> MDYKDDDDKLAAANSSIDLISTSLYKKAGLTMVTGGGAAPPGTVTEPLPSVIVLSAGRKMAAAAAAASGPGCSSAAGAGAAGVSEWLVLRDGCMHCDADGLHSLSYHPALNAILAVTSRGTIKVIDGTSGATLQASALSAKPGGQVKCQYISAVDKVIFVDDYAVGCRKDLNGILLLDTALQTPVSKQDDVVQLELPVTEAQQLLSACLEKVDISSTEGYDLFITQLKDGLKNTSHETAANHKVAKWATVTFHLPHHVLKSIASAIVNELKKINQNVAALPVASSVMDRLSYLLPSARPELGVGPGRSVDRSLMYSEANRRETFTSWPHVGYRWAQPDPMAQAGFYHQPASSGDDRAMCFTCSVCLVCWEPTDEPWSEHERHSPNCPFVKGEHTQNVPLSVTLATSPAQFPCTDGTDRISCFGSGSCPHFLAAATKRGKICIWDVSKLMKVHLKFEINAYDPAIVQQLILSGDPSSGVDSRRPTLAWLEDSSSCSDIPKLEGDSDDLLEDSDSEEHSRSDSVTGHTSQKEAMEVSLDITALSILQQPEKLQWEIVANVLEDTVKDLEELGANPCLTNSKSEKTKEKHQEQHNIPFPCLLAGGLLTYKSPATSPISSNSHRSLDGLSRTQGESISEQGSTDNESCTNSELNSPLVRRTLPVLLLYSIKESDEKAGKIFSQMNNIMSKSLHDDGFTVPQIIEMELDSQEQLLLQDPPVTYIQQFADAAANLTSPDSEKWNSVFPKPGTLVQCLRLPKFAEEENLCIDSITPCADGIHLLVGLRTCPVESLSAINQVEALNNLNKLNSALCNRRKGELESNLAVVNGANISVIQHESPADVQTPLIIQPEQRNVSGGYLVLYKMNYATRIVTLEEEPIKIQHIKDPQDTITSLILLPPDILDNREDDCEEPIEDMQLTSKNGFEREKTSDISTLGHLVITTQGGYVKILDLSNFEILAKVEPPKKEGTEEQDTFVSVIYCSGTDRLCACTKGGELHFLQIGGTCDDIDEADILVDGSLSKGIEPSSEGSKPLSNPSSPGISGVDLLVDQPFTLEILTSLVELTRFETLTPRFSATVPPCWVEVQQEQQQRRHPQHLHQQHHGDAAQHTRTWKLQTDSNSWDEHVFELVLPKACMVGHVDFKFVLNSNITNIPQIQVTLLKNKAPGLGKVNALNIEVEQNGKPSLVDLNEEMQHMDVEESQCLRLCPFLEDHKEDILCGPVWLASGLDLSGHAGMLTLTSPKLVKGMAGGKYRSFLIHVKAVNERGTEEICNGGMRPVVRLPSLKHQSNKGYSLASLLAKVAAGKEKSSNVKNENTSGTRKSENLRGCDLLQEVSVTIRRFKKTSISKERVQRCAMLQFSEFHEKLVNTLCRKTDDGQITEHAQSLVLDTLCWLAGVHSNGPGSSKEGNENLLSKTRKFLSDIVRVCFFEAGRSIAHKCARFLALCISNGKCDPCQPAFGPVLLKALLDNMSFLPAATTGGSVYWYFVLLNYVKDEDLAGCSTACASLLTAVSRQLQDRLTPMEALLQTRYGLYSSPFDPVLFDLEMSGSSCKNVYNSSIGVQSDEIDLSDVLSGNGKVSSCTAAEGSFTSLTGLLEVEPLHFTCVSTSDGTRIERDDAMSSFGVTPAVGGLSSGTVGEASTALSSAAQVALQSLSHAMASAEQQLQVLQEKQQQLLKLQQQKAKLEAKLHQTTAAAAAAASAVGPVHNSVPSNPVAAPGFFIHPSDVIPPTPKTTPLFMTPPLTPPNEAVSVVINAELAQLFPGSVIDPPAVNLAAHNKNSNKSRMNPLGSGLALAISHASHFLQPPPHQSIIIERMHSGARRFVTLDFGRPILLTDVLIPTCGDLASLSIDIWTLGEEVDGRRLVVATDISTHSLILHDLIPPPVCRFMKITVIGRYGSTNARAKIPLGFYYGHTYILPWESELKLMHDPLKGEGESANQPEIDQHLAMMVALQEDIQCRYNLACHRLETLLQSIDLPPLNSANNAQYFLRKPDKAVEEDSRVFSAYQDCIQLQLQLNLAHNAVQRLKVALGASRKMLSETSNPEDLIQTSSTEQLRTIIRYLLDTLLSLLHASNGHSVPAVLQSTFHAQACEELFKHLCISGTPKIRLHTGLLLVQLCGGERWWGQFLSNVLQELYNSEQLLIFPQDRVFMLLSCIGQRSLSNSGVLESLLNLLDNLLSPLQPQLPMHRRTEGVLDIPMISWVVMLVSRLLDYVATVEDEAAAAKKPLNGNQWSFINNNLHTQSLNRSSKGSSSLDRLYSRKIRKQLVHHKQQLNLLKAKQKALVEQMEKEKIQSNKGSSYKLLVEQAKLKQATSKHFKDLIRLRRTAEWSRSNLDTEVTTAKESPEIEPLPFTLAHERCISVVQKLVLFLLSMDFTCHADLLLFVCKVLARIANATRPTIHLCEIVNEPQLERLLLLLVGTDFNRGDISWGGAWAQYSLTCMLQDILAGELLAPVAAEAMEEGTVGDDVGATAGDSDDSLQQSSVQLLETIDEPLTHDITGAPPLSSLEKDKEIDLELLQDLMEVDIDPLDIDLEKDPLAAKVFKPISSTWYDYWGADYGTYNYNPYIGGLGIPVAKPPANTEKNGSQTVSVSVSQALDARLEVGLEQQAELMLKMMSTLEADSILQALTNTSPTLSQSPTGTDDSLLGGLQAANQTSQLIIQLSSVPMLNVCFNKLFSMLQVHHVQLESLLQLWLTLSLNSSSTGNKENGADIFLYNANRIPVISLNQASITSFLTVLAWYPNTLLRTWCLVLHSLTLMTNMQLNSGSSSAIGTQESTAHLLVSDPNLIHVLVKFLSGTSPHGTNQHSPQVGPTATQAMQEFLTRLQVHLSSTCPQIFSEFLLKLIHILSTERGAFQTGQGPLDAQVKLLEFTLEQNFEVVSVSTISAVIESVTFLVHHYITCSDKVMSRSGSDSSVGARACFGGLFANLIRPGDAKAVCGEMTRDQLMFDLLKLVNILVQLPLSGNREYSARVSVTTNTTDSVSDEEKVSGGKDGNGSSTSVQGSPAYVADLVLANQQIMSQILSALGLCNSSAMAMIIGASGLHLTKHENFHGGLDAISVGDGLFTILTTLSKKASTVHMMLQPILTYMACGYMGRQGSLATCQLSEPLLWFILRVLDTSDALKAFHDMGGVQLICNNMVTSTRAIVNTARSMVSTIMKFLDSGPNKAVDSTLKTRILASEPDNAEGIHNFAPLGTITSSSPTAQPAEVLLQATPPHRRARSAAWSYIFLPEEAWCDLTIHLPAAVLLKEIHIQPHLASLATCPSSVSVEVSADGVNMLPLSTPVVTSGLTYIKIQLVKAEVASAVCLRLHRPRDASTLGLSQIKLLGLTAFGTTSSATVNNPFLPSEDQVSKTSIGWLRLLHHCLTHISDLEGMMASAAAPTANLLQTCAALLMSPYCGMHSPNIEVVLVKIGLQSTRIGLKLIDILLRNCAASGSDPTDLNSPLLFGRLNGLSSDSTIDILYQLGTTQDPGTKDRIQALLKWVSDSARVAAMKRSGRMNYMCPNSSTVEYGLLMPSPSHLHCVAAILWHSYELLVEYDLPALLDQELFELLFNWSMSLPCNMVLKKAVDSLLCSMCHVHPNYFSLLMGWMGITPPPVQCHHRLSMTDDSKKQDLSSSLTDDSKNAQAPLALTESHLATLASSSQSPEAIKQLLDSGLPSLLVRSLASFCFSHISSSESIAQSIDISQDKLRRHHVPQQCNKMPITADLVAPILRFLTEVGNSHIMKDWLGGSEVNPLWTALLFLLCHSGSTSGSHNLGAQQTSARSASLSSAATTGLTTQQRTAIENATVAFFLQCISCHPNNQKLMAQVLCELFQTSPQRGNLPTSGNISGFIRRLFLQLMLEDEKVTMFLQSPCPLYKGRINATSHVIQHPMYGAGHKFRTLHLPVSTTLSDV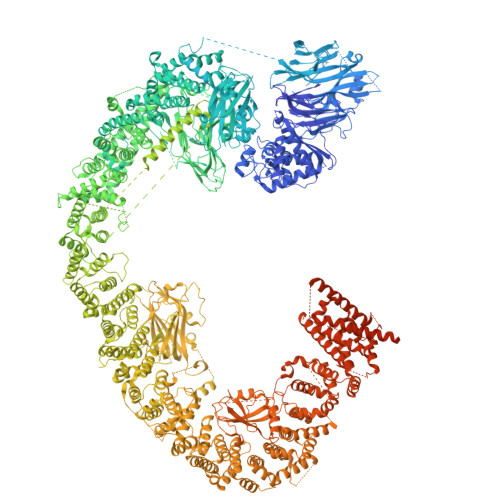LDRVSDTPSITAKLISEQKDDKEKKNHEEKEKVKAENGFQDNYSVVVASGLKSQSKRAVSATPPRPPSRRGRTIPDKIGSTSGAEAANKIITVPVFHLFHKLLAGQPLPAEMTLAQLLTLLYDRKLPQGYRSIDLTVKLGSRVITDPSLSKTDSYKRLHPEKDHGDLLASCPEDEALTPGDECMDGILDESLLETCPIQSPLQVFAGMGGLALIAERLPMLYPEVIQQVSAPVVTSTTQEKPKDSDQFEWVTIEQSGELVYEAPETVAAEPPPIKSAVQTMSPIPAHSLAAFGLFLRLPGYAEVLLKERKHAQCLLRLVLGVTDDGEGSHILQSPSANVLPTLPFHVLRSLFSTTPLTTDDGVLLRRMALEIGALHLILVCLSALSHHSPRVPNSSVNQTEPQVSSSHNPTSTEEQQLYWAKGTGFGTGSTASGWDVEQALTKQRLEEEHVTCLLQVLASYINPVSSAVNGEAQSSHETRGQNSNALPSVLLELLSQSCLIPAMSSYLRNDSVLDMARHVPLYRALLELLRAIASCAAMVPLLLPLSTENGEEEEEQSECQTSVGTLLAKMKTCVDTYTNRLRSKRENVKTGVKPDASDQEPEGLTLLVPDIQKTAEIVYAATTSLRQANQEKKLGEYSKKAAMKPKPLSVLKSLEEKYVAVMKKLQFDTFEMVSEDEDGKLGFKVNYHYMSQVKNANDANSAARARRLAQEAVTLSTSLPLSSSSSVFVRCDEERLDIMKVLITGPADTPYANGCFEFDVYFPQDYPSSPPLVNLETTGGHSVRFNPNLYNDGKVCLSILNTWHGRPEEKWNPQTSSFLQVLVSVQSLILVAEPYFNEPGYERSRGTPSGTQSSREYDGNIRQATVKWAMLEQIRNPSPCFKEVIHKHFYLKRVEIMAQCEEWIADIQQYSSDKRVGRTMSHHAAALKRHTAQLREELLKLPCPEGLDPDTDDAPEVCRATTGAEETLMHDQVKPSSSKELPSDFQL>[2x]TPEKEPLKPGDILVYAQGGGEPKPIRLEELKPGDPFVLAYPMDPKTKVVKSGEAKNTLLVARFDPEELAPEVAQHAAEGVVAYSAVCTHLGCIV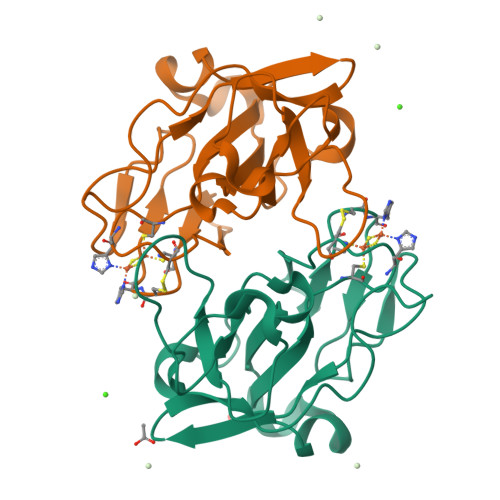SQWVADEEAALCPCHGGVYDLRHGAQVIAGPPPRPVPQLPVRVEDGVLVAAGEFLGPVGVQA> MEESKTLKSENHEPKKNVICEESKAVQVIGNQTLKARNDKSVKEIENSSPNRNSSKKNKQNDICIEKTEVKSCKVNAANLPGPKDLGLVLRDQSHCKAKKFPNSPVKAEKATISQAKSEKATSLQAKAEKSPKSPNSVKAEKASSYQMKSEKVPSSPAEAEKGPSLLLKDMRQKTELQQIGKKIPSSFTSVDKVNIEAVGGEKCALQNSPRSQKQQTCTDNTGDSDDSASGIEDVSDDLSKMKNDESNKENSSEMDYLENATVIDESALTPEQRLGLKQAEERLERDHIFRLEKRSPEYTNCRYLCKLCLIHIENIQGAHKHIKEKRHKKNILEKQEESELRSLPPPSPAHLAALSVAVIELAKEHGITDDDLRVRQEIVEEMSKVITTFLPECSLRLYGSSLTRFALKSSDVNIDIKFPPKMNHPDLLIKVLGILKKNVLYVDVESDFHAKVPVVVCRDRKSGLLCRVSAGNDMACLTTDLLTALGKIEPVFIPLVLAFRYWAKLCYIDSQTDGGIPSYCFALMVMFFLQQRKPPLLPCLLGSWIEGFDPKRMDDFQLKGIVEEKFVKWECNSSSATEKNSIAEENKAKADQPKDDTKKTETDNQSNAMKEKHGKSPLALETPNRVSLGQLWLELLKFYTLDFALEEYVICVRIQDILTRENKNWPKRRIAIEDPFSVKRNVARSLNSQLVYEYVVERFRAAYRYFACPQTKGGNKSTVDFKKREKGKISNKKPVKSNNMATNGCILLGETTEKINAEREQPVQCDEMDCTSQRCIIDNNNLLVNELDFADHGQDSSSLSTSKSSEIEPKLDKKQDDLAPSETCLKKELSQCNCIDLSKSPDPDKSTGTDCRSNLETESSHQSVCTDTSATSCNCKATEDASDLNDDDNLPTQELYYVFDKFILTSGKPPTIVCSICKKDGHSKNDCPEDFRKIDLKPLPPMTNRFREILDLVCKRCFDELSPPCSEQHNREQILIGLEKFIQKEYDEKARLCLFGSSKNGFGFRDSDLDICMTLEGHENAEKLNCKEIIENLAKILKRHPGLRNILPITTAKVPIVKFEHRRSGLEGDISLYNTLAQHNTRMLATYAAIDPRVQYLGYTMKVFAKRCDIGDASRGSLSSYAYILMVLYFLQQRKPPVIPVLQEIFDGKQIPQRMVDGWNAFFFDKTEELKKRLPSLGKNTESLGELWLGLLRFYTEEFDFKEYVISIRQKKLLTTFEKQWTSKCIAIEDPFDLNHNLGAGVSRKMTNFIMKAFINGRKLFGTPFYPLIGREAEYFFDSRVLTDGELAPNDRCCRVCGKIGHYMKDCPKRKSLLFRLKKKDSEEEKEGNEEEKDSRDVLDPRDLHDTRDFRDPRDLRCFICGDAGHVRRECPEVKLARQRNSSVAAAQLVRNLVNAQQVAGSAQQQGDQSIRTRQSSECSESPSYSPQPQPFPQNSSQSAAITQPSSQPGSQPKLGPPQQGAQPPHQVQMPLYNFPQSPPAQYSPMHNMGLLPMHPLQIPAPSWPIHGPVIHSAPGSAPSNIGLNDPSIIFAQPAARPVAIPNTSHDGHWPRTVAPNSLVNSGAVGNSEPGFRGLTPPIPWEHAPRPHFPLVPASWPYGLHQNFMHQGNARFQPNKPFYTQDRCATRRCRERCPHPPRGNVSE;> MGSVSNQQFAGGCAKAAEEAPEEAPEDAARAADEPQLLHGAGICKWFNVRMGFGFLSMTARAGVALDPPVDVFVHQSKLHMEGFRSLKEGEAVEFTFKKSAKGLESIRVTGPGGVFCIGSERRPKGKSMQKRRSKGDRCYNCGGLDHHAKECKLPPQPKKCHFCQSISHMVASCPLKAQQGPSAQGKPTYFREEEEEIHSPTLLPEAQN

Tumor-suppressor let-7 pre-microRNAs (miRNAs) are regulated by terminal uridylyltransferases TUT7 and TUT4 that either promote let-7 maturation by adding a single uridine nucleotide to the pre-miRNA 3′ end or mark them for degradation by the addition of multiple uridines. Oligo-uridylation is increased in cells by enhanced TUT7/4 expression and especially by the RNA-binding pluripotency factor LIN28A. TUT4 and TUT7 are multidomain enzymes whose specific targeting of RNAs makes use of three zinc fingers, combined with two copies of a nucleotidyltransferase domain (NTD), one inactive in the N-terminal half of the polypeptide (pseudo-NTD) and one active in the C-terminal half. Our structures reveal that pre-miRNAs engage the enzymes in fundamentally different ways depending on the presence of LIN28A, which clamps them onto the TUTs to enable processive 3′ oligo-uridylation.

To compare with TUT7, a truncated TUT4 (residues 254–1315) with a similar activity to the full-length TUT4 protein and to an N-terminal-only truncated form (residues 153–1649) was expressed and purified from the E. coli KRX strain and assembled with LIN28A and pre-let-7g before polishing by size-exclusion chromatography. A 3.68 Å cryo-EM structure was obtained for the TUT4/LIN28A/pre-let-7 in the pre-oligo-uridylation capture state found also as TUT7 ternary conformation I. This structure enabled us to identify more clearly the interactions between the LIM module of TUT4, LIN28A and the pre-let-7. Although the CM of TUT4 is not well defined in the 3D map, density apparently derived from it can be visualized in two-dimensional (2D) class averages of the complex, roughly oriented in the same view compared to the TUT4 ternary complex in conformation I, in line with this being a capture state before CM engagement with the open end of the pre-let-7g. The 49AGGAG53 recognition sequence from pre-let-7g was observed trapped into a positively charged pocket created by TUT4 and LIN28A. Together with the TUT7 ternary complexes this structure therefore provides a demonstration that TUT4 interacts directly with LIN28A, a currently unresolved and key question in the field. In this ternary interface, a hydrophobic patch is formed between G276, L277, A280, I316 from TUT4 LIM (which are conserved in TUT7: G216, L217, A220, I256) and prolines 156 and 168 of LIN28A. The pre-let-7g is observed bound to three main interfaces in the TUT4 capture complex, which we have termed interface 1, interface 2 and interface 3, respectively. Interface 3 is critical to the ternary interaction: in this region the zinc finger of the TUT4 LIM is observed to bind the 49AGGAG53 region of pre-let-7 and the two ZKs of LIN28A. The side chains of four positively charged residues R283, R286, H320 and K324 from the LIM participate in the interaction with G51, A52, G53 and A54 of the pre-let-7g.>[2x]MADPWQECMDY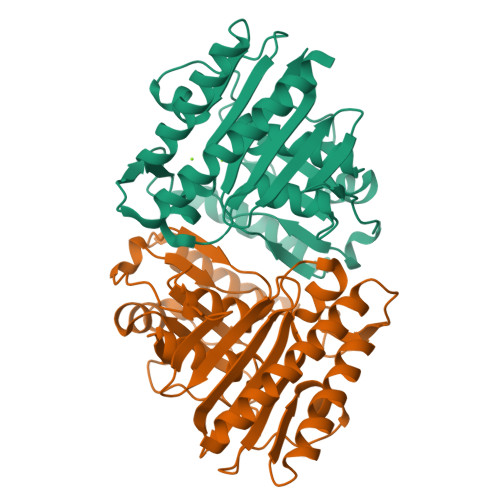AVTLAGQAGEVVREALKNEMNIMVKSSPADLVTATDQKVEKMLITSIKEKYPSHSFIGEESVAAGEKSILTDNPTWIIDPIDGTTNFVHGFPFVAVSIGFVVNKKMEFGIVYSCLEDKMYTGRKGKGAFCNGQKLQVSHQEDITKSLLVTELGSSRTPETVRIILSNIERLLCLPIHGIRGVGTAALNMCLVAAGAADAYYEMGIHCWDVAGAGIIVTEAGGVLLDVTGGPFDLMSRRVIASSNKTLAERIAKEIQIIPLQRDDED> SMQEEDTFRELRIFLRNVTH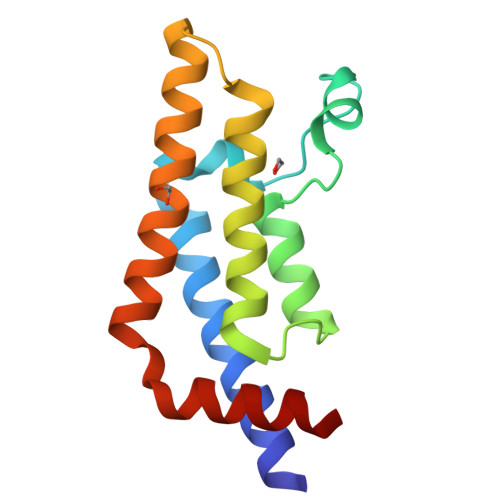RLAIDKRFRVFTKPVDPDEVPDYRTVIKEPMDLSSVISKIDLHKYLTVKDYLRDIDLICSNALEYNPDRDPGDRLIRHRACALRDTAYAIIKEELDEDFEQLCEEIQESR>GPAMEKYEGDWVNGKMHGHGKYIYSDGGVYEGDWIDGKMHGKGTYVFPNGNVYEGEWAHDMKDGYGVLTYQNGEKYEGYWKQDKVHGKGTLTYTRGDKYIGDWMDAKKDGEGELIYANGDRFKGQWADDRANGFGVFTYANGNRYEGEWTDDKRHGRGVFYCAEDGSAYEGEFVGGRKEGNGILRLATGHQLEGTWSGGQLVRVTSFVFAQDSPWLNVDL[2x]

High-resolution crystal structures and biophysical analyses of a truncated form of the TbMORN1 protein and its homologues from the parasites Toxoplasma gondii (TgMORN1) and Plasmodium falciparum (PfMORN1) enabled, for the first time, a structure-based definition of the MORN repeat. All three structures are antiparallel dimers joined via their C-termini, and, when possessed of the correct key residues, can adopt extended or V-shaped quaternary structures. The crystal structures confirmed that each 23-amino acid MORN repeat is composed of a β-hairpin followed by a 6-residue loop that connects to the next MORN repeat. The structural studies presented here make a case that one conserved function of MORN repeats is in homotypic interactions and possibly also in higher-order assembly.

The structures of TgMORN1(7–15) and both P21 and C2 crystal forms of TbMORN1(7–15) were subsequently determined to 2.90, 2.35 and 2.53 Å resolution, respectively, with the PfMORN1(7–15) structure used as a search model for the molecular replacement. The two subunits in the TbMORN1(7–15) C2 crystal form and the TgMORN1(7–15) dimer make a rather straight assembly, while in the P21 form they display a bend of about 30°, leading to a rod-shaped particle appearance. TbMORN1(7–15) formed an extended antiparallel dimer in both crystal lattices, while TgMORN1(7–15) adopted this architecture in one crystal form. In comparison to the TbMORN1(7–15) C2 crystal form, the extended TgMORN1(7–15) structure has an approximately 1.5-times smaller dimer interface (601 Å2), which is contributed by residues from MORN repeats 13–15 only. This is closer in size to the 747 Å2 interface of the P21 crystal form of TbMORN1(7–15). The final C-terminal part of the protein seems to be flexible and does not engage in the stabilisation of the dimer. In comparison to TbMORN1(7–15), the dimer interface of TgMORN1(7–15) is not built around aromatic stacking but instead employs hydrophobic interactions between Phe350 and neighbouring small hydrophobic residues, such as Leu335 and Leu327. In contrast to TbMORN1(7–15), where the dimerisation interface is centred around aromatic stacking, a hydrophobic core plays a crucial role in the dimer interface of extended TgMORN1(7–15). The dimer is stabilised by a single salt bridge formed between the Asp308 of one subunit and the His333 of the other subunit. SAXS analysis of TbMORN1(7–15) and TgMORN1(7–15) indicated an extended dimer in solution and the crystal structures could be docked into the calculated molecular envelopes without difficulty.> AL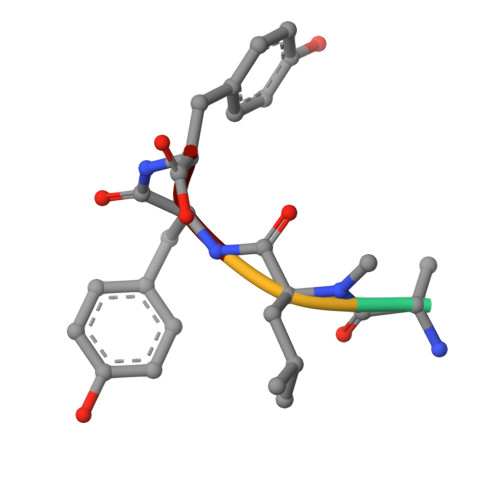YY> TDTTNSIKHVISPLARQTLQDRDLTRPVAGKRPIRLLPWLQVVKIGGRVMDRGADAILPLVEELRKLLPEHRLLILTGAGVRARHVFSVGLDLGLPVGSLA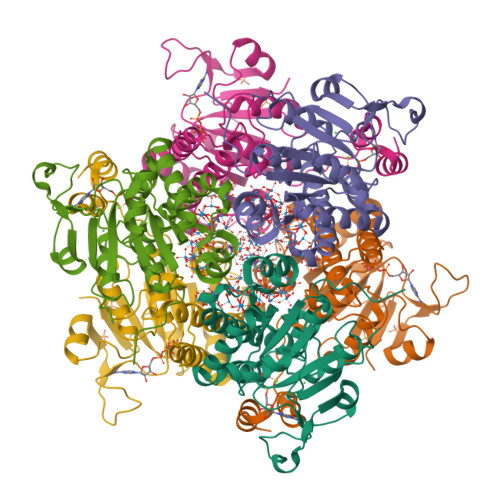PLAASEAGQNGHILAAMLASEGVSYVEHPTVADQLAIHLSATRAVVGSAFPPYHHHEFPGSRIPPHRADTGAFLLADAFGAAGLTIVENVDGIYTADPNGPDRGQARFLPETSATDLAKSEGPLPVDRALLDVMATARHIERVQVVNGLVPGRLTAALRGEHVGTLIRTGVRPA;> ANSTAELEELLMQRSLTDPQLQAAAAAAADFRILPDATVIKIGGQSVIDRGRAAVYPLVDEIVAARKNHKLLIGTGAGTRARHLYSIAAGLGLPAGVLAQLGSSVADQNAAMLGQLLAKHGIPVVGGAGHSAVPLSLAEVNAVVFSGMPPYKLWMRPAAEGVIPPYRTDAGCFLLAEQFGCKQMIFVKDEDGLYTANPKTSKDATFIPRISVDEMKAKGLHDSILEFPVLDLLQSAQHVREVQVVNGLVPGNLTRALAGEHVGTIITAS>[2x]TIKVGINGFGRIGRIVFRAAQKRSDIEIVAINDLLDADYMAYMLKYDSTHGRFDGTVEVKDGHLIVNGKKIRVTAERDPANLKWDEVGVDVVAEATGLFLTDETARKHITAGAKKVVMTGPSKDNTPMFVKGANFDKYAGQDIVSNASCTTNCLAPLAKVINDNFGIIEGLMTTVHATTATQKTVDGPSHKDWRGGRGASQNIIPSSTGAAKAVGKVLPELNGKLTG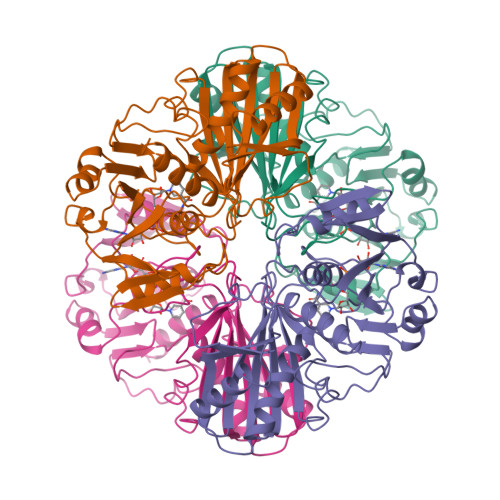MAFRVPTPNVSVVDLTVRLEKAATYEQIKAAVKAAAEGEMKGVLGYTEDDVVSTDFNGEVCTSVFDAKAGIALNDNFVKLVSWYDTETGYSNKVLDLIAHISK>MLSGLNHLTLAVSQLAPSVAFYQQLLGMTLHARWDSGAYLSCGDLWLCLSLDPQRRVTPPEESDYTHYAFSISEADFASFAARLEAAGVAVWKLNRSEGASHYFLDPDGHKLELHVGSLAQRLAACREQPYKGMVFFEQHHHHHH[2x]

Here we systematically compare RT fragment screening of the Fosfomycin-resistance protein A from Klebsiella pneumoniae (FosAKP), an enzyme involved in antibiotic resistance, with conventional single crystal data collection at cryogenic temperature (cryo). Fosfomycin, a broad-spectrum antibiotic, is routinely used to treat urinary infections. However, natural resistance can exist in gram-negative bacteria, mainly through the enzyme Fosfomycin-resistance protein A (FosA), that catalyzes the Mn2+ and K+-dependent glutathione mediated inactivation of Fosfomycin. Therefore, increased interest exists to identify inhibitors of FosA to enable the use of Fosfomycin to also treat resistant strains24.

Over all screens, a total of 31 out of 95 fragments are observed binding to FosAKP. For comparison, the same screen was conducted with conventional single crystal data collection at cryogenic temperatures (100 K) from loop-mounted crystals at beamline P11 at PETRA III. In total, 7 fragments bind in the two RT screens, of which 3 bind to pharmaceutically relevant sites 1, 2 and 4. In contrast, 31 fragments are observed binding in the cryo screens, but only 6 of these bind to the more interesting sites 1-4.> ETPPRFTRTPVDQTGVSGGVASFICQATGDPRPKIVWNKKGKKVSNQRFEVIEFDDGSGSVLRIQPLRTPRDEAIYECVASNNVGEISVSTRLTVLREDQIPRGFPTIDMGPQLKVVERTRTATMLCAASGNPDPEITWFKDFLPVDTSNNNGRIKQLRSESIGGTPIRGALQIEQSEESDQGKYECVATNSAGTRYSAPANLYVRELREVRRVPPRFSIPPTNHEIMPGGSVNITCVA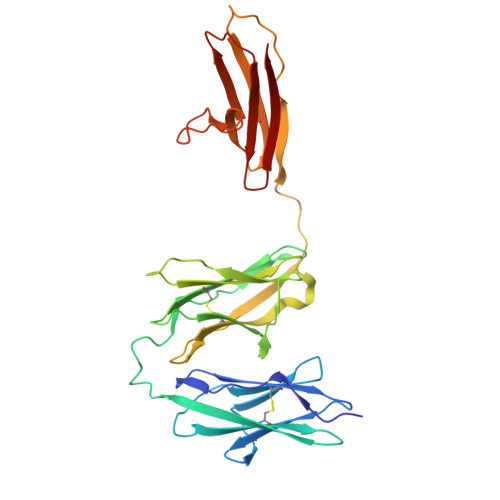VGSPMPYVKWMLGAEDLTPEDDMPIGRNVLELNDVRQSANYTCVAMSTLGVIEAIAQIT>MNVTIYDVAREASVSMATVSRVVNGNPNVKPSTRKKVLETIERLGYRPNAVARGLASKKTTTVGVIIPDISNIFYAELARGIEDIASMYKYNIILSNSDQNQDKQLHLLNNMLGKQVDGIIFMSGNVTEEHVEELKKSPVPVVLAASIESTNQIPSVTIDYEQAAFDAVQSLIDSGHKNIAFVSGTLEEPINHAKKVKGYKRALTESGLPVRDSYIVEGDYTYDSGIEAVEKLLEEDEKPTAIFVGTDEMALGVIHGAQDRGLNVPNDLEIIGFDNTRLSTMVRPQLTSVVQPMYDIGAVAMRLLTKYMNKETVDSSIVELPHRIEFRQSTK[3x];>[3x]MVQQKVEVRLKTGLQARPAALFVQEANRFTSDIFLEKDGKKVNAKSIMGLMSLAISTGTEI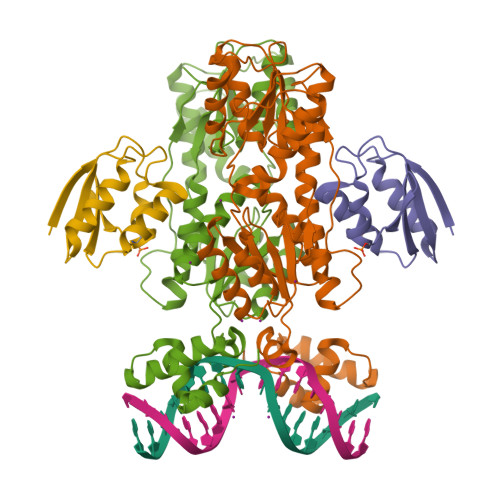TLIAQGEDEQEALEKLAAYVQEEV> MILDTDYITENGKPVIRVFKKENGEFKIEYDRTFEPYFYALLKDDSAIEDVKKVTAKRHGTVVKVKRAEKVQKKFLGRPIEVWKLYFNHPQDVPAIRDRIRAHPAVVDIYEYDIPFAKRYLIDKGLIPMEGDEELTMLAFAIATLYHEGEEFGTGPILMISYADGSEARVITWKKIDLPYVDVVSTEKEMIKRFLRVVREKDPDVLITYNGDNFDFAYLKKRCEELGIKFTLGRDGSEPKIQRMGDRFAVEVKGRIHFDLYPVIRRTINLPTYTLEAVYEAVFGKPKEKVYAEEIAQAWESGEGLERVARYSMEDAKVTYELGREFFPMEAQLSRLIGQSLWDVSRSSTGNLVEWFLLRKAYKRNELAPNKPDERELARRRGGYAGGYVKEPERGLWDNIVYLDFRSLYPSIIITHNVSPDTLNREGCKEYDVAPEVGHKFCKDFPGFIPSLLGDLLEERQKIKRKMKATVDPLEKKLLDYRQRLIKILANSFYGYYGYAKARWYCKECAESVTAWGREYIEMVIRELEEKFGFKVLYADTDGLHATIPGADAETVKKKAKEFLKYINPKLPGLLELEYEGFYVRGFFVTKKKYAVIDEEGKITTRGLEIVRRDWSEIAKETQARVLEAILKHGDVEEAVRIVKEVTEKLSKYEVPPEKLVIHEQITRDLRDYKATGPHVAVAKRLAARGVKIRPGTVISYIVLKGSGRIGDRAIPADEFDPTK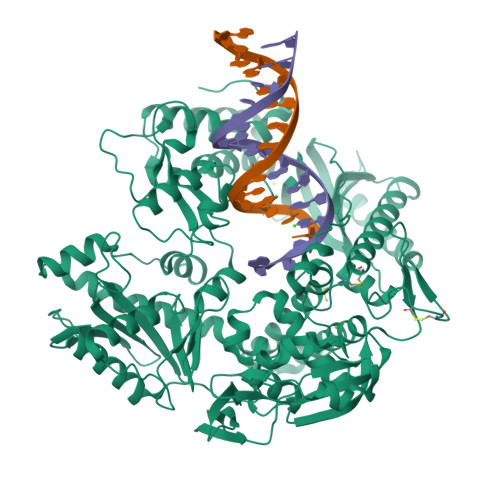HRYDAEYYIENQVLPAVERILKAFGYRKEDLRYQKTKQVGLGAWLKVKGKKLEHHHHHH>[2x]AEFWNEYEDFRSFFKKKFGKDLTGYQRLWAKRIVQGKSFTMVAPTGVGKTTFGMMTALWLARKGKKSALVFPTVTLVKQTLERLQKLADEKVKIFGFYSSMKKEEKEKFEKSFEEDDYHILVFSTQFVSK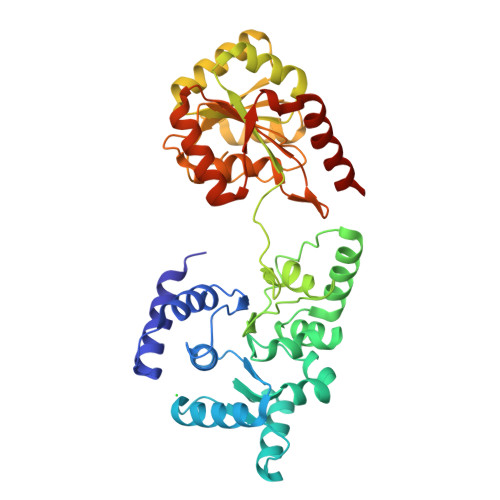NREKLSQKRFDFVFVDDVDAVLKASRNIDTLLMMVGIPEEIIRKAFSTIKQGKIYERPKNLKPGILVVSSATAKPRGIRPLLFRDLLNFTVGRLVSVARNITHVRISSRSKEKLVELLEIFRDGILIFAQTEEEGKELYEYLKRFKFNVGETWSEFEKNFEDFKVGKINILIGVQAYYGKLTRGVDLPERIKYVIFWGTPSGPDVYTYIQASGRSSRILNGVLVKGVSVIFEEDEEIFESLKTRLLLIAEEEIIEEAEANWKELVHEVEESRRRSERELTDTSR> TRSGK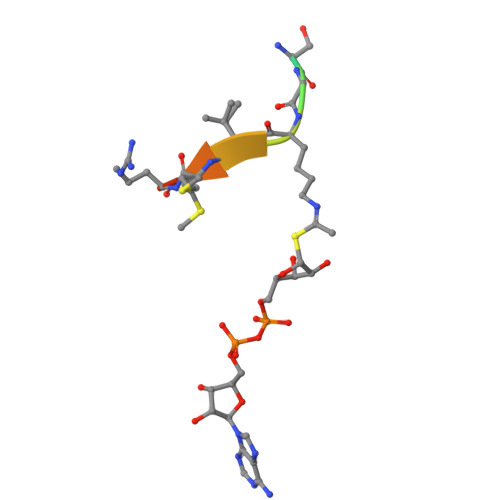VMRRL>GPAMLPISMSDEGDSFLVKDSLGENKIPKNPSKVVILDLGILDTFDALKLNDKVVGVPAKNLPKYLQQFKNKPSVGGVQQVDFEAINALKPDLIIISGRQSKFYDKLKEIAPTLFVGLDNANFLSSFENNVLSVAKLYGLEKEALEKISDIKNEIEKAKSIVDEDKKALIILTNSNKISAFGPQSRFGIIHDVLG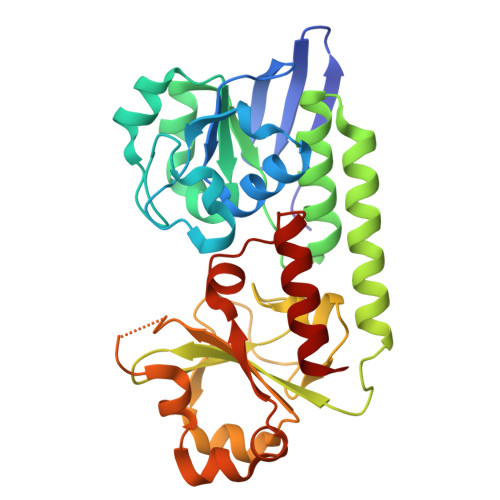INAVDENIKVGTAGKSINSEFILEKNPDYIFVVDRNVILGNKERAQGILDNALVAKTKAAQNKKIIYLDPEYWYLASGNGLESLKTMILEIKNAVK[3x]SARS and related coronaviruses and astroviruses all possess a motif at the 3′ end of their RNA genomes, called the s2m, whose pathogenic importance is inferred from its rigorous sequence conservation in an otherwise rapidly mutable RNA genome. The viral replicase is translated directly from the genomic sense-strand RNA, and it then creates a full-length complementary (minus-sense strand) copy of the genomic RNA, as well as a nested set of shorter, subgenomic mRNAs having common 3′ UTRs. These 3′ UTRs all share with the genomic SARS RNA a 32-nucleotide element, immediately upstream of the 3′ poly-A tail (residues 29,590–29,621), originally termed the stem-loop II motif (s2m) in human astroviruses. The s2m element is the most highly conserved RNA element within the coronaviruses and astroviruses that contain it. We find that this extreme conservation is clearly explained by the requirement to form a highly structured RNA whose unique tertiary structure includes a sharp 90° kink of the helix axis and several novel longer-range tertiary interactions.

Using in vitro transcription, we prepared and crystallized a 48-nucleotide construct containing the 45-nucleotide s2m element. We solved the crystal structure to 2.7-Å resolution using a single platinum isomorphous/anomalous derivative and obtained a readily interpretable solvent-flattened electron density map. The overall structure of the s2m SARS RNA consists of two regions that are defined by two perpendicular RNA helix axes. The larger region contains several non-helical motifs involved in long-range tertiary contacts. The smaller region (residues 20–30, shown in yellow in Figure 3) forms a stem-loop structure in which a pentaloop (residues 22–26) is structured similar to a conventional GNRA tetraloop motif but has an extra residue (U) bulged out of the stack formed by A(23), G(24), A(26), and the augmenting helical stem (residues 20–21 and 27–28). Although the structure of the pentaloop is very similar to the standard GNRA tetraloop structure, the “extra” U(25) insertion between R and A is always present. The unusual perpendicular helical junction is stabilized by the formation of an RNA base quartet involving two adjacent G–C pairs wherein the G(19)/C(31) pair shares four hydrogen bonds with the C(20)/G(28) pair (shown as pink dotted lines in Figure 3A and 3B). A(17) pairs with G(34), involving the Watson–Crick base-pairing faces of both purines. As a consequence, A(33) is able to adopt a very unusual conformation in which it becomes completely excluded from the helical stack, and instead forms long-range tertiary interactions with G(11) and A(12). A base triple forms between A(38) and this G–C pair, a variant of the adenosine platform motif, and consequently G(11) and A(12) are rotated out of the helical structure completely.

> GGAGUUCACCGAGGCCACGCGGAGUACGAUCGAGGGUACAGUGAAUU>MAHHHHHHMAISPRDEQNRSVDLWFAYKVPKLTK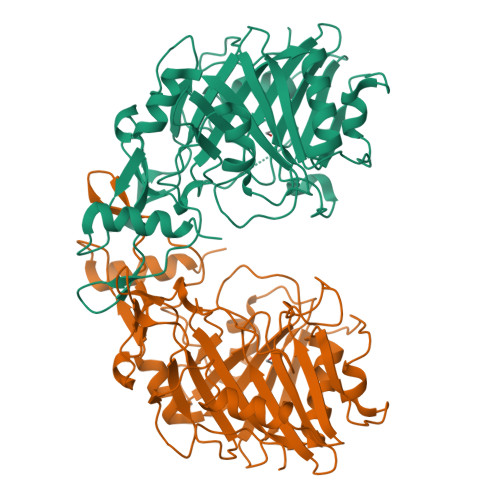DADSDSASGYEYVYYDRQVGAVQKSPNLMNDPKGALFYTLDSVFGDPGDTTGWILYNDEMPADANRSNNATLGHTKGVIAFDIASSSALWLLHSWPKYASPSVPGVPTPLYGQTFLCLSLDLATAGKLAAQMALHQQPQVYLPRTGGLDHTSPLYALTQPLNASAPGDSDSLDFKTRGGVPFKVIAKNRKWGKDFWNDLVGPTLKADMYVETWIRGKIPPVLDSDGVHKTYDIKFIDLRKLGAPWAWPETQDHAKWGITTTDNWVCVGDINRMVTQEKRGGGTIAFQDPKLWKALCETDLIIPPPGKTDAQARAMIRKTHEPAE[2x]> MAKNTSITLGEHFDGFI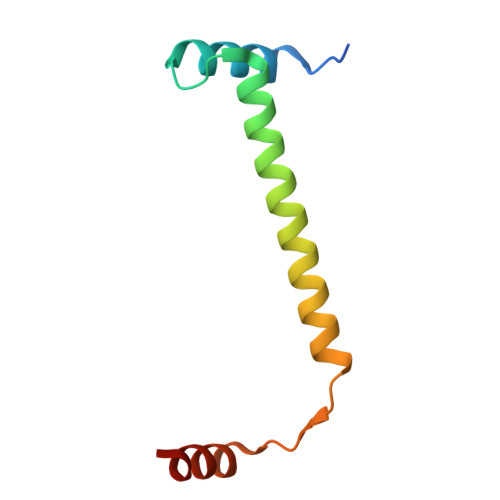TSQIQSGRYGSASEVIRSALRLLENQETKLQSLRQLLIEGEQSGDADYDLDSFINELDSENIR> 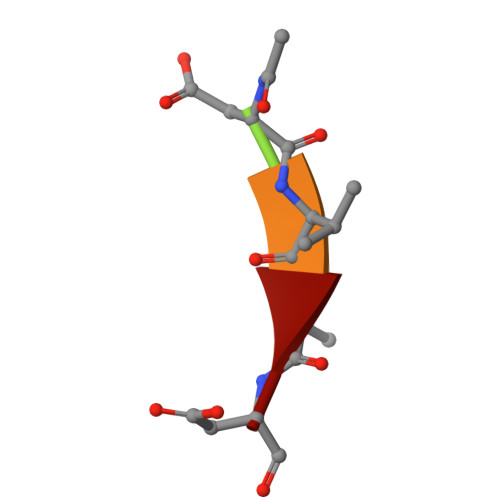XDVAD N-hexanoyl-L-homoserine | C10 H19 N O4 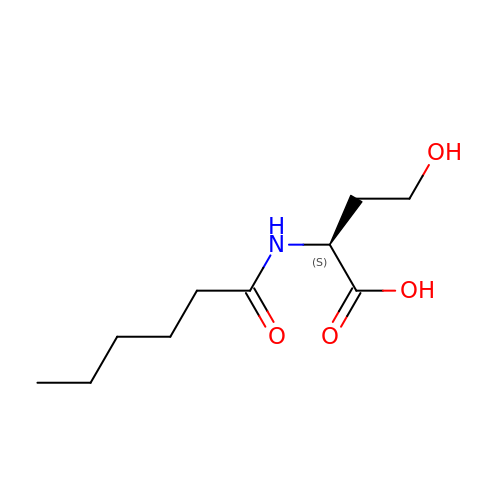| BJLILZXVIKTHKQ-QMMMGPOBSA-N> SSNFNQETVTDIHHWTDTLFSFRTTRDPGFRFQSGQFIMMGLEVNGKPLTRAYSIASSLYEDGLEFFSIKVPNGPLTSKLQHLKKGDQIIVSKKPVGTLLYDNLKPGKHLWLLSTGTGLAPFL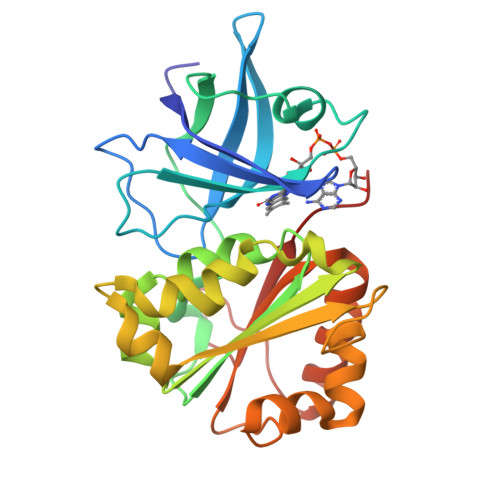SIIRDLEVYERFEKVILVHGVRQVAELAYTDFISNELPQDEFLGEMVKNQLIYYPTVTREPYKTRGRLTDLIRSGQLFKDVGLPEFNHEDDRMMLCGSPEMLAETKQILEERGFTEGSQSEPGEFVIEKAFVEK> MGHHHHHHGNSRSRVGRSFCSQFLPEEQAEIDQLFDALSSDKNSPNVSSKSFSLKALQNHVGEALPPEMVTRLYDGMRRVDLTGKAKGPSENVSQEQFTASMSHLLKGNSEEKSLMIMKMISATEGPVKAREVQKFTEDLVGSVVHVLSHRQELRGWTGKEAPGPNPRVQVLAAQLLSDMKLQDGKRLLGPQWLDYDCDRAVIEDWVFRVPHVAIFLSVVICKGFLVLC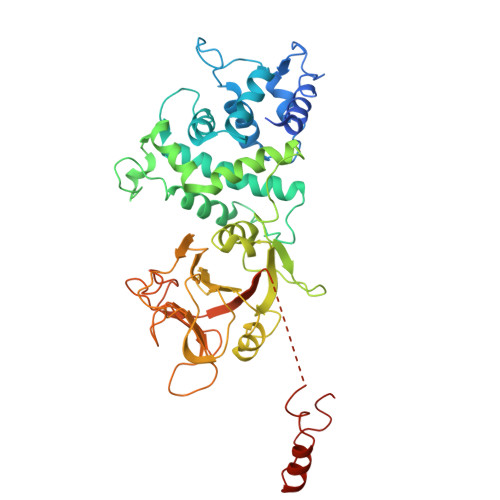SSLDLTTLVPERQVDQGRGFESILDVLSVMYINAQLPREQRHRWRLLFSSELHGHSFSQLCGHITHRGPCVAVLEDHDKHVFGGFASCSWEVKPQFQGDNRCFLFSICPSMAVYTHTGYNDHYMYLNHGQQTIPNGLGMGGQHNYFGLWVDVDFGKGHSRAKPTCTTYNSPQLSAQENFQFDKMEVWAVGDPSEEQLAKGNKSILDADPEAQALLEISGHSRHSEGLREVPDDE>[3x]SNAKELNDLEKKYNAHIGVYALNTKSGKEVKFNSDKRFAYASTSKAINSAILLEQVPYNKLNKKVHINKDDIVAYSPILEKYVGKDITLKELIEASMTYSDNTANNKIIKEIGGIKKVKQ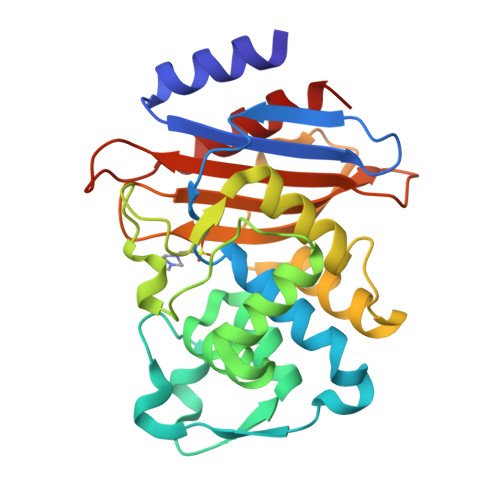RLKELGDKVTNPVRYEIELNYYSPKSKKDTSTPAAFGKTLNKLIANGKLSKKNKNFLLDLMFNNKNGDTLIKDGVPKDYKVADKSGQAITYASRNDVAFVYPKGQSEPIVLVIFTNKDNKSDKPNDKLISETAKSVMKEF>[2x]MAEQVKPAGVKPKGTVPPPKGNAPAPKANGAPGGASVIKEQDAAKMRRFLFQRTETRSTKWYQIFDTEKLDDEQVVGGHLALLGVLGFIMGIYYISGIQVFPWGAPGFHDNWFYLTIKPRMVSLGIDTYSTKTADLEAAGARLLGWAAFHFLVGSVLIFGGWRHWTHNLTNPFTGRCGNFRDFRFLGKFGDVVFNGTSAKSYKEALGPHAVYMSLLFLGWGIVMWAILGFAPIPDFQTINSETFMSFVFAVIFFALGIYWWNNPPNAAIHLNDDMKAAFSVHLTAIGYINIALGCIA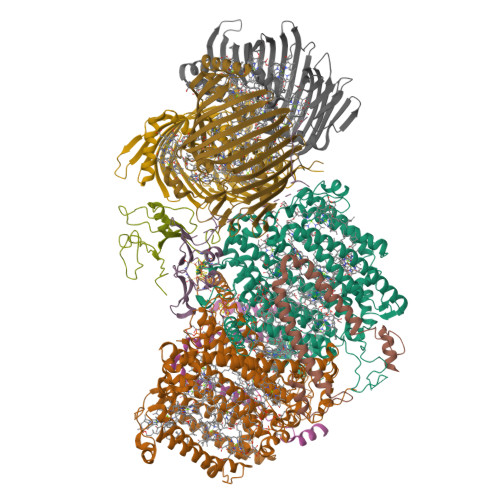FVAFQQPSFAPYYKELDKLVFYLYGEPFNRVSFNFVEQGGKVISGAKEFADFPAYAILPKSGEAFGMARVVTNLIVFNHIICGVLYVFAGVYHGGQYLLKIQLNGMYNQIKSIWITKGRDQEVQVKILGTVMALCFATMLSVYAVIVWNTICELNIFGTNITMSFYWLKPLPIFQWMFADPSINDWVMAHVITAGSLFSLIALVRIAFFAHTSPLWDDLGLKKNSYSFPCLGPVYGGTCGVSIQDQLWFAMLWGIKGLSAVCWYIDGAWIASMMYGVPAADAKAWDSIAHLHHHYTSGIFYYFWTETVTIFSSSHLSTILMIGHLVWFISFAVWFEDRGSRLEGADIQTRTIRWLGKKFLNRDVNFRFPVLTISDSKLAGTFLYFGGTFMLVFLFLANGFYQTNSPLPPPVSHAAVSGQQMLAQLVDTLMKMIA;> MAEPVENKNQAPAPGAKVPPKGAPAAPKAGAPAAPKGPVAPKAGAPAAKTGASAAKQAGKPRLASLGVTLGRSGVRQESALPYVKPKAVPPPKPAAPAAKGAPAPKGAPAAPAAKAAPGAPVAKAAPKAKKHYFIIENLCVGCGLCLDKCPPKVNAIGYKFYGDVQEGGFRCYIDQAACISCSACFSGDECPSGALIEVLPDGEVLDFSYTPPERLDFDLRFLHRFHREAR;>MDKNSNGKLIALAVGGAVLMGALFFSVSFLTGYIPAPNHSAILTPLRSFMGWFLLIFCASIIIMGLGKMSSAISDKWFLSFPLSIFVIVMVMFLSLRVYWEKGRTTTVDGKYIRTTAELKEFLNKPAATSDVPPAPAGFDFDAAKKLVDVRCNKCHTLDSVADLFRTKYKKTGQVNLIVKRMQGFPGSGISDDDAKTIGIWLHEKF[2x];> MQPQLSRPQTASNQVRKAVSGPWSGNAVHKAEKYFITSAKRDRDGKLQIELVPASGRRKLSPTPEMIRRLIDGEIEIYILTTQPDIAIDMNKEIIDMENRYVIDFDKRGVKWTMREIPVFYHEGKGLCVELHNKIYTLDQFFK;>[3x]MALFGSNDVTTAHSDYEIVLEGGSSSWGKVKARAKVNAPPASPLLPADCDVKLNVKPLDPAKGFVRISAVFESIVDSTKNKLTIEADIANETKERRISVGEGMVSVGDFSHTFSFEGSVVNLFYYRSDAVRRNVPNPIYMQGRQFHDILMKVPLDNNDLIDTWEGTVKAIGSTGAFNDWIRDFWFIGPAFTALNEGGQRISRIEVNGLNTESGPKGPVGVSRWRFSHGGSGMVDSISRWAELFPSDKLNRPAQVEAGFRSDSQGIEVKVDGEFPGVSVDAGGGLRRILNHPLIPLVHHGMVGKFNNFNVDAQLKVVLPKGYKIRYAAPQYRSQNLEEYRWSGGAYARWVEHVCKGGVGQFEILYAQ> RSKKGDKNGKGLRHFSMKVCEKVQRKGTTSYNEVADELVSEFTNSNNHL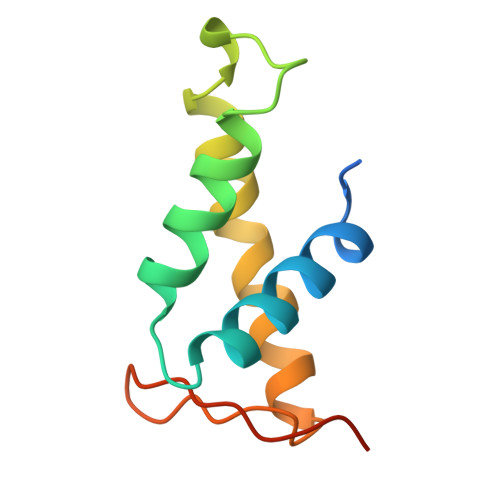AADSAYDQKNIRRRVYDALNVLMAMNIISKEKKEIKWIGLPTNSAQ2-ethoxyphenol | C8 H10 O2 | 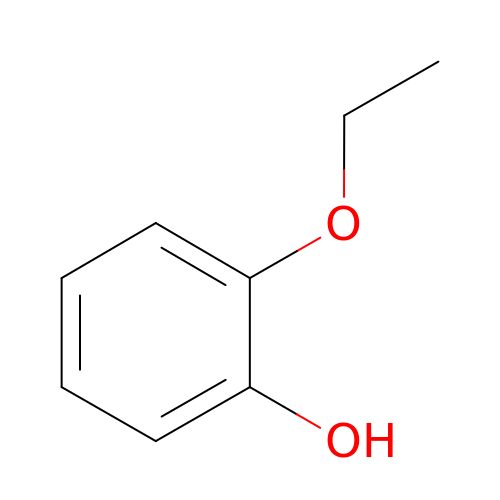MOEFFSWKSMRFRQ-UHFFFAOYSA-N> AGFIDDSTLTGGIYYWQRERDRKDLNPDSKDYNQYTTNLSHSTANLSLDFASGYAWDMFGLDVGAFTAIELAESSASGHPNEIAFSSKNRTYDEDYS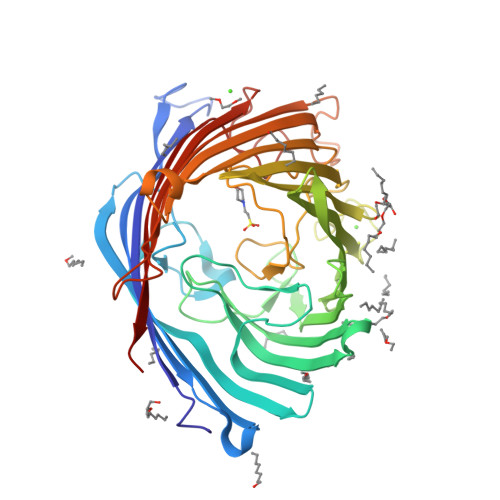GDKGGVSLYKAAAKFKYGPVWARAGYIQPSGQTLLAPHWSFMPGTYQGAEAGAKFDYGDAGALSFSYMWADKYKAPWHIEVDDFRQNDKKTRVSYLHSLGAKYDFKNDLVLEAAFGQAQGYVNQYFTKASYKFDVLGNPLTTSYQFYGAEDRISDKNDPNSIYDGLAWLQALTFGYTTGQFNWRLEGTMVKAEGNQGFFLQRMTPTYASSNGRLDVWWDNRSDFNANGEKAVYAGVMYDLSNWNLPGMAVGGSYVYAWDAKPSTNPIYDQSQRLKESAWSLDAMYTIQEGRAKGTLIKLHYTQYDNHTNIPSWGGGYGNIFQDEKDVKFMVIAPFTIF1-(AMINOETHYL)AMINO-4-AMINOBUTANE | C6 H17 N3 | 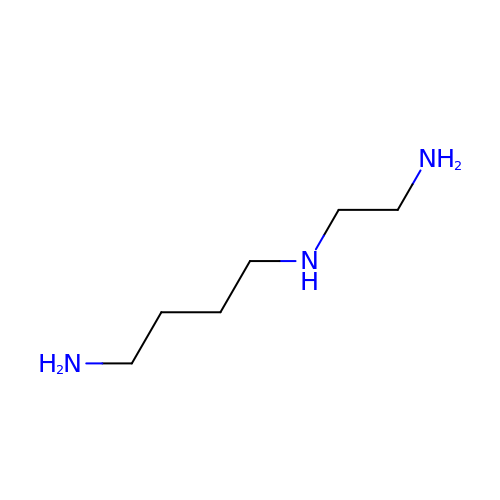VRPPEXGZBZBARW-UHFFFAOYSA-N> GSHHHHHHSSGTENLYFQENFILYEEIGRGSKTVVYKGRRKGTINFVAILCTDKCKRPEITNWVRLTREIKHKNIVTFHEWYETSNHLWLVVELCTGGSLKTVIAQDENLPEDVVREFGIDLISGLHHLHKLGILFCDISPRKILLEGPGTLKFSNFCLAKVEGENL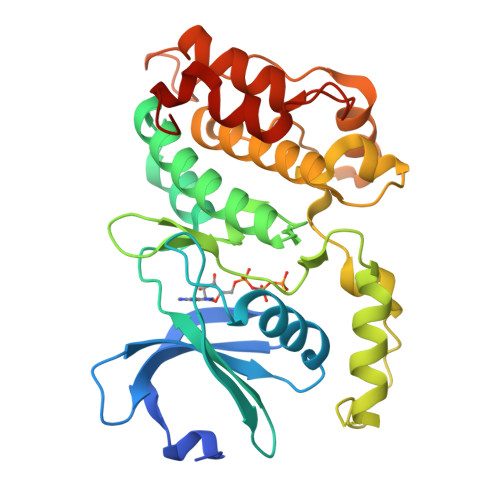EEFFALVAAEEGGGDNGENVLKKSMKSRVKGSPVYTAPEVVRGADFSISSDLWSLGCLLYEMFSGKPPFFSESISELTEKILCEDPLPPIPKDSSRPKASSDFINLLDGLLQRDPQKRLTWTRLLQHSFWKKAFAGAD> MKFLLLSALLFLHSSLAWTREKHYYIGITEAVWDYASGSEEKELISVDTEQSNFYLRNGPDRIGRKYKKALYSEYTDGTFTKTIDKPAWLGLLGPVIKAEVGDKVSVHVKNFASRPYTFHAHGVTYTKANEGAIYPDNTTDFQRADDKLFPGQQYLYVLRANEPSPGEGDSNCVTRIYHSHVDAPKDIASGLIGPLILCKKGSLHKEKEENIDQEFVLMFSVVDENLSWYLEDNIKTFCSEPEKVDKDNEDFQESNRMYSINGYTFGSLPGLSMCAEDRVKWYLFGMGNEVDVHSALFHGQALTSKNYHTDIINLFPATLIDVSMVAQNPGVWMLSCQNLNHLKAGLQAFFQVRDCNKPSPDDDIQDRHVRHYYIAAEETIWDYAPSGTDTFTGENLTSLGSDSRVFFEQGATRIGGSYKKLVYREYTDDSFTNRKQRGPDEEHLGILGPVIWAEVGDIIRVTFHNKGQFPLSIQPMGVRFTKENEGTYYGPDGRSSKQASHVAPKETFTYEWTVPKEMGPTYADPVCLSKMYYSGVDLTKDIFTGLIGPMKICKKGSLLADGRQKDVDKEFYLFATVFDENESLLLDDNIRMFTTAPENVDKEDEDFQESNKMHSMNGFMYGNLPGLNMCLGESIVWYLFSAGNEADVHGIYFSGN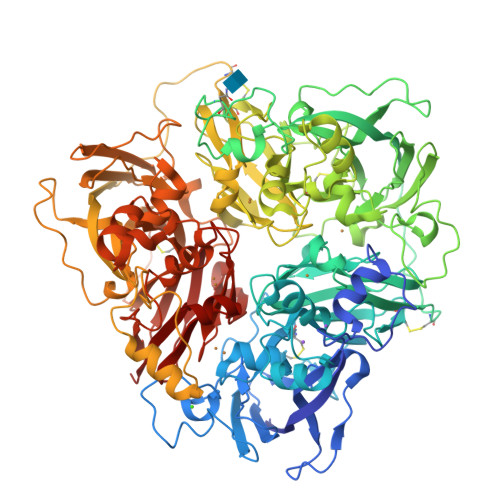TYLSKGERRDTANLFPHKSLTLLMTPDTEGSFDVECLTTDHYTGGMKQKYTVNQCKGQFEDVTLYQGERTYYIAAVEVEWDYSPSRDWEMELHHLQEQNVSNAFLDKEEFFIGSKYKKVVYREFTDSTFREQVKRRAEEEHLGILGPLIHADVGDKVKVVFKNMASRPYSIHAHGVKTKSSTVAPTLPGEVRTYIWQIPERSGAGTEDSPCIPWAYYSTVDRVKDLYSGLIGPLIVCRKSYVKVFNPKKKMEFSLLFLVFDENESWYLDDNINTYSDHPEKVNKDNEEFIESNKMHAINGKMFGNLQGLTMHVGDEVNWYVMAMGNEIDLHTVHFHGHSFQYKHRGIHSSDVFDLFPGTYQTLEMFPQTPGTWLLHCHVTDHIHAGMVTTYTVLPNQETKSG(2Z)-N-biphenyl-4-yl-2-cyano-3-cyclopropyl-3-hydroxyprop-2-enamide | C19 H16 N2 O2 | 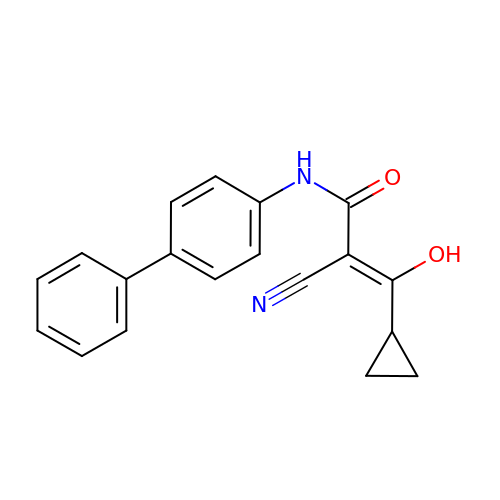CAGGGMPTWTUYHZ-ZCXUNETKSA-N> MAQDALSDGFVRLCIDPSLNFFGEGCKILVEGQITDDATAAENVVTCVNSELDLVERFGQGSVLTESLRKVFCMCKSGVSVYALPRADAAAAVSAVYTLTVTGTALTDGRVQLYMGEAEYSLDIGVDEGDTPTQIAAKIVAAISPDFPYEATAAAGVITLTARNGGTIGNHLSVIYTNLGSCTSVTPEGVTVAFAQTTPGSVNPEPNDYASVVNECCFAVYVLSSDDTDWQENLRDWIRSAWDCSKPQCFGHGYVFNKGTLGQVLADGDNSAELSRLALPTTYPVLPYLTNAAYGALSACSTCENPELNVQGQTYGLLSCINMPESCTPGWEFTEVTQLQNNGFVVSGPAT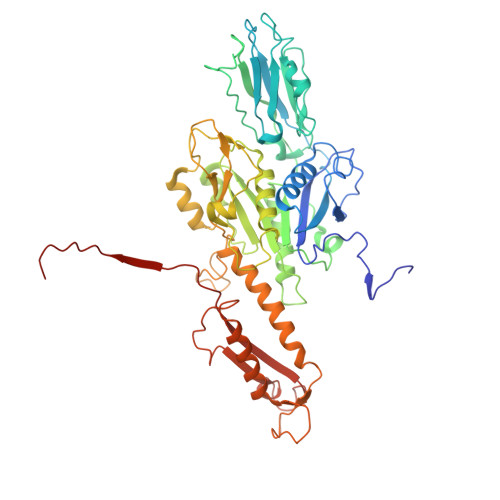TSGQGNFTSPYIYNDVTNYLRDEKNRPNATFRDASSRRLAAATGVALATFLQQFNGLAVFTKNTNIKTGIIGTNLRLMLGKIRKWASDNVGVLFSEFDNINEDIQLVSDFDVQPKCVGQPGVFHLNMRYRPPVRGARINVNLVPALFDNCDR>MFEIKKICCIGAGYVGGPTCSVIAHMCPEIRVTVVDVNESRINAWNSPTLPIYEPGLKEVVESCRGKNLFFSTNIDDAIKEADLVFISVNTPTKTYGMGKGRAADLKYIEACARRIVQNSNGYKIVTEKSTVPVRAAESIRRIFDANTKPNLNLQVLSNPEFLAEGTAIKDLKNPDRVLIGGDETPEGQRAVQALCAVYEHWVPREKILTTNTWSSELSKLAANLFLAQRISSINSISALCEATGADVEEVATAIGMDQRIGNKFLKASVGFGGSCFQKDVLNLVYLCEALNLPEVARYWQQVIDMNDYQRRRFASRIIDSLFNTVTDKKIAILGFAFKKDTGDTRESSSIYISKYLMDEGAHLHIYDPKVPREQIVVDLSHPGVSEDDQVSRLVTI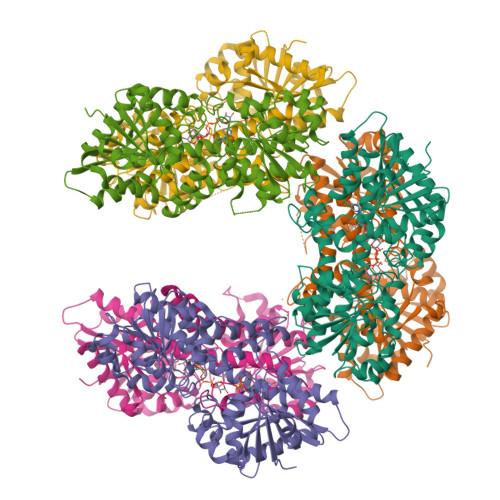SKDPYEACDGAHAVVICTEWDMFKELDYERIHKKMLKPAFIFDGRRVLDGLHNELQTIGFQIETIGKKVSSKRIPYAPSGEIPKFSLQDPPNKKPKV[6x]> MREWKIIDSTLREGEQFEKANFSTQDKVEIAKALDEFGIEYIEVTTPVASPQSRKDAEVLASLGLKAKVVTHIQCRLDAAKVAVETGVQGIDLLFGTSKYLRAPHGRDIPRIIEEAKEVIAYIREAAPHVEVRFSAEDTFRSEEQDLLAVYEAVAPYVDRVGLADTVGVATPRQVYALVREVRRVVGPRVDIEFHGHNDTGCAIANAYEAIEAGATHVDTTIL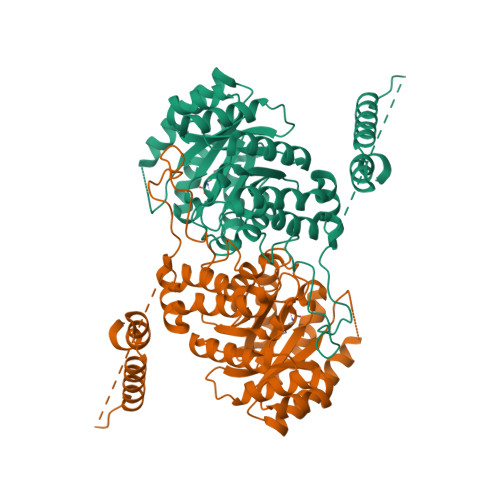GIGERNGITPLGGFLARMYTLQPEYVRRKYKLEMLPELDRMVARMVGVEIPFNNYITGETAFSHKAGMHLKAIYINPEAYEPYPPEVFGVKRKLIIASRLTGRHAIKARAEELGLHYGEEELHRVTQHIKALADRGQLTLEELDRILREWITA> GDALRLARRIAAALNASDNNAGDYGFFWITAVTTDGSIVVANSYGLAYIPDGMELPNKVYLASADHAIPVDEIARCATYPVLAVQAWA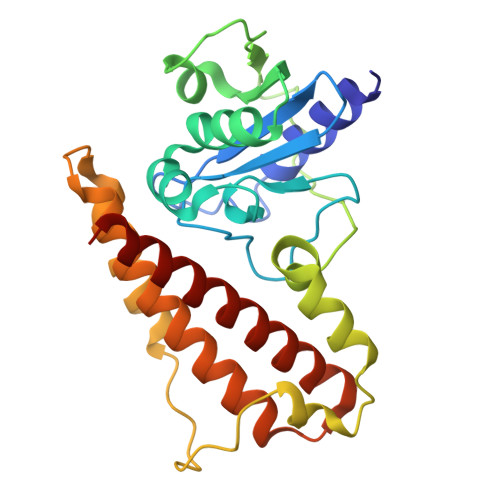AFHDMTLRAVIGTAEQLASSDPGVAKIVLEPDDIPESGKMTGRSRLEVVDPSAAAQLADTTDQRLLDLLPPAPVDVNPPGDERHMLWFELMKPMTSTATGREAAHLRAFRAYAAHSQEIALHQAHTATDAAVQRVAVADWLYWQYVTGLLDRALAAAC> KPRKVWIIYSADHPLYVDVVLKFAQFLLTACGTEVALDLLEEQAISEAGVMTWVGRQKQEMVESNSKIIVLCSRGTRAKWQALLGRGAPVRLRCDHGKPVGDLFTAAMNMILPDFKRPACFGTYVVCYFSEVSCDGDVPDLFGAAPRYPLMDRFEEVYFRIQDLEMFQPGRMHRVGELSGDNYLRSPGGRQLRAALDRFRDWQVRCPDWFECENLY

A unique intracellular signaling domain termed SEFIR is found within all IL-17 receptors (IL-17Rs) as well as the key adaptor protein Act1. SEFIR-mediated protein–protein interaction is a crucial step in IL-17 cytokine signaling. The IL-17 receptor (IL-17R) family comprises five members (IL-17RA to IL-17RE) with considerable sequence divergence, which are all membrane-bound proteins containing single transmembrane domains. IL-17Rs contain fibronectin type III (FnIII) domains within the extracellular portion and a unique structural motif within the cytoplasmic tails termed the SEFIR [SEF (similar expression to fibroblast growth factor genes) and IL-17R] domain.

Here, we report the crystal structure of a fragment from the IL-17RA intracellular signaling domain including its SEFIR domain and a short C-extension at 2.3 Å resolution. Besides the complete SEFIR domain (residues 376–540) of IL-17RA, the structure reported here additionally includes a short C-terminal extension (residues 556–591) of about 35 amino acids. The structure is well defined except for two flexible loops, the electron densities of which are not observable. One is a six-amino-acid short linker (residues 471–476) within the CC′ loop. The other is a 14-amino-acid linker (residues 541–555) connecting helices αE and αE′. The longer helix αF is sandwiched by two short helices, αE′ and αG, in a Z-shaped crank shape. This predominantly helical C-extension of SEFIR packs tightly against helices αA and CC′ins and loops CC′, DD′ and EE′ through extensive van der Waals interactions, stabilizing the overall architecture. In contrast to the complete disorder in the structure of IL-17RB SEFIR, the unique and long insertion between strand βC and helix αC in the IL-17RA SEFIR structure is mostly well ordered, displaying a helix (αCC′ins) and a flexible loop (CC′). The most striking observation when comparing the two SEFIR structures is the absence of the knot feature in IL-17RA SEFIR. The DD′ loop in IL-17RA SEFIR is much shorter compared with that in IL-17RB SEFIR. Together with the short helix αD, it rotates almost 90° with respect to the IL-17RB SEFIR structure and shifts by more than 12 Å, making sufficient space to accommodate the αCC′ins helix. The results here implicate that the αC helix of IL-17RA is the most critical region within the SEFIR domain for its heterotypic interaction with Act1 and is essential for IL-17A signaling.In humans, NEET proteins are represented by MiNT, localized inside the mitochondria, mitoNEET, and NAF-1, both anchored to the mitochondria outer membrane; with NAF-1 being also present on the surface of the endoplasmic reticulum and its mitochondria-associated membrane. NEET proteins harbor two [2Fe-2S] clusters with a unique 3Cys:1His coordination structure. Indeed, a growing amount of evidence demonstrate that NEET proteins play a significant role in Fe/Fe-S exchange between mitochondria and cytosol in cells. Here we report, for the first time, on a chemical compound, M1, that accelerates the dissociation of the [2Fe–2S] clusters of mNT and NAF-1 in a dose dependent manner.

M1-mNT structure determined by X-ray crystallography at 1.65 Å resolution shows the presence of an extra density that correspond to M1 molecule on each mNT monomer; monomer A and monomer B (respectively). According to the M1-mNT structure, M1 is in close proximity to the [2Fe–2S] cluster binding domain where the tetralin ring of M1 is oriented toward the [2Fe–2S] cluster while the distal phenyl ring is facing the β-cap domain. The M1 carboxyl group forms a salt bridge with Lys55 (2.2 Å distance between them) but it does not interact with His87 (3.5 and 3.7 Å distance). M1 is also oriented towards the side chain of Lys68 (β-cap domain of mNT) and forms a hydrogen bond with it (2.9 Å distance). Moreover, the surface of mNT and NAF-1 show hydrophobic residues facing the hydrophobic moieties of M1 (<4.5 Å) suggesting hydrophobic interactions between M1 and the mNT/NAF-1 protein. M1 binds strongly to the Lys55/Lys81 in mNT/NAF-1, respectively. In the native protein, hydrogen bond formation between Lys55/Lys81 and His87/His114 (mNT/NAF-1), is critical for cluster stability with His87/His114 in effect performing a gatekeeper function which is compromised upon M1 binding to Lys55/Lys81 to result in higher lability of the bound clusters. Previous studies indicated that Lys68 mutagenesis (insertion at this position) destabilizes mNT’s [2Fe–2S] clusters. Taken together the structures of M1-mNT/NAF-1 strongly suggest that in addition to His87/His114, interactions with Lys55/81 and cross-talk between the β-cap and the cluster binding area are also playing an important role in mNT and NAF-1 cluster lability/stability.

>RFYVKDHRNKAMINLHIQKDNPKIVHAFDMEDLGDKAVYCRCWRSKKFPFCDGAHTKHNEETGDNVGPLIIKKKET[2x]>[2x]METPLLELIAIVRQGSEEQQKSALEQLKRLLEAGADPNAADNAGKTPLLLLIEIVRQGSEEQQKAALELLKLLLEAGADPNAADNAGKTPLLLLIEIVRQGSEEQQKAALELLKLLLEAG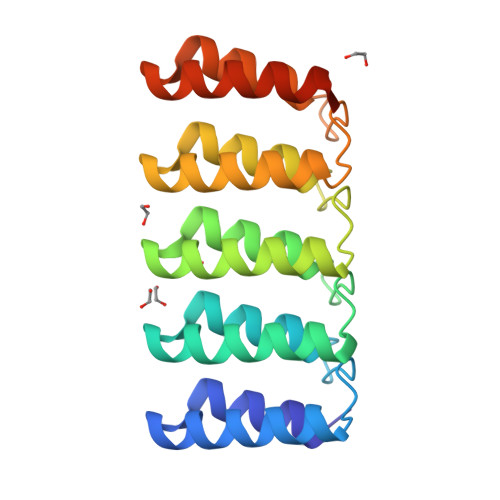ADPNAADNAGKTPLLLLIEIVRQGSEEQQKAALELLKLLLEAGADPNAADNAGQTPQQLLKAIERQGSEEQQKAAKELLKLLEEAGGSWGHHHHHH>[2x]AMAGVFTYETEFTSVIPPPRLFKAFILDAD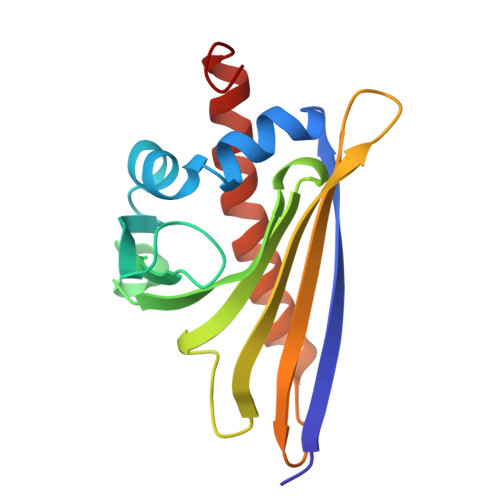NLIPKIAPQAVKCAEIIEGDGGVGTIKKITFGEGSQFGSVTHKIDGIDKENFVYSYSLIEGDALSDKIEKISYETKLVSSSDGGSIIKSTSNYHTKGDVEIKEEHVKAGKEKFSHLFKLVEGYLLANPNEYC At the axonal surface, type IIa receptor protein tyrosine phosphatases (RPTPs) (type IIa RPTPs, for example, RPTPσ, RPTPδ and leukocyte common antigen-related (LAR) in vertebrates, dLAR in Drosophila), are a recently identified nexus for extracellular interactions, receiving signals and transmitting them intracellularly to the cytoskeleton to regulate neuronal extension and guidance, as well as synaptic organization. There are two major neuronal RPTPσ isoforms, sharing a common intracellular catalytic region and an extracellular region predicted to contain three immunoglobulin (Ig)-like domains followed by either five or nine fibronectin (FN) type III domains, in the central and peripheral nervous systems, respectively. Previous mutagenesis and structural studies have demonstrated that the proteoglycan-binding site lies on Ig1 of RPTPσ, and comprises an extended positively charged surface of basic residues101314. Binding of postsynaptic TrkC, is reported to require the N-terminal three Ig domains of RPTPσ17; the NGL-3-binding site has been mapped to the FN1-2 domains.

We reveal that the multi-domain extracellular region of RPTPσ is unexpectedly flexible. We determined the 3.15 Å crystal structure of a six N-terminal domain human RPTPσ construct (termed Ig1-FN3), which contains all the binding sites for synaptic ligands identified to date. This construct maintains the V-shaped Ig1–2 arrangement previously reported, followed by an extended conformation of the sequential domains Ig3, FN1 and FN2. While FN1 and FN2 domains align approximately with the long axis of the molecule, the C-terminal FN3 domain folds back, suggesting the FN2-3 linker may also be a flexion point. Since no substantial Ig3-FN1, FN1–FN2 or FN2–FN3 inter-domain interfaces are apparent, we hypothesized that when released from crystal packing constraints each of the Ig2-FN3 region linkers may provide substantial flexibility. To test this, single-particle negative-stain electron microscopy (EM) class averages of human RPTPσ Ig1-FN3 were calculated. These showed a broad range of conformations. To control for the potential risk of artefacts associated with negative staining, we also performed small-angle X-ray scattering (SAXS) measurements, at a physiological pH (7.4), for both human RPTPσ Ig1-FN3 and sEcto. This analysis further supports the observation that both proteins are flexible and are likely to adopt multiple conformations in solution. Taken together, crystallographic, EM and SAXS analyses demonstrate that the ectodomain of RPTPσ is able to explore a large conformational space.

> ETGEEPPRFIKEPKDQIGVSGGVASFVCQATGDPKPRVTWNKKGKKVNSQRFETIEFDESAGAVLRIQPLRTPRDENVYECVAQNSVGEITVHAKLTVLREDQLPSGFPNIDMGPQLKVVERTRTATMLCAASGNPDPEITWFKDFLPVDPSASNGRIKQLRSGALQIESSEETDQGKYECVATNSAGVRYSSPANLYVRVRRVAPRFSILPMSHEIMPGGNVNITCVAVGSPMPYVKWMQGAEDLTPEDDMPVGRNVLELTDVKDSANYTCVAMSSLGVIEAVAQITVKSLPKAPGTPMVTENTATSITITWDSGNPDPVSYYVIEYKSKSQDGPYQIKEDITTTRYSIGGLSPNSEYEIWVSAVNSIGQGPPSESVVTRTGEQAPASAPRNVQARMLSATTMIVQWEEPVEPNGLIRGYRVYYTMEPEHPVGNWQKHNVDDSLLTTVGSLLEDETYTVRVLAFTSVGDGPLSDPIQVKTQQGVPGQPMNLRAEARSETSITLSWSPPRQESIIKYELLFREGDHGREVGRTFDPTTSYVVEDLKPNTEYAFRLAARSPQGLGAFTPVVRQRTLGTKHHHHHH>MPILEKAPQKMPVKASSWEELDLPKLPVPPLQQTLATYLQCMQHLVPEEQFRKSQAIVKRFGAPGGLGETLQEKLLERQEKTANWVSEYWLNDMYLNNRLALPVNSSPAVIFARQHFQDTNDQLRFAACLISGVLSYKTLLDSHSLPTDWAKGQLSGQPLCMKQYYRLFSSYRLPGHTQDTLVAQKSSIMPEPEHVIVACCNQFFVLDVVINFRRLSEGDLFTQLRKIVKMASNEDERLPPIGLLTSDGRSEWAKARTVLLKDSTNRDSLDMIERCICLVCLDGPGTGELSDTHRALQLLHGGGCSLNGANRWYDKSLQFVVGRDGTCGVVCEHSPFDGIVLVQCTEHLLKHMMTSNKKLVRADSVSELPAPRRLRWKCSPETQGHLASSAEKLQRIVKNLDFIVYKFDNYGKTFIKKQKYSPDGFIQVALQLA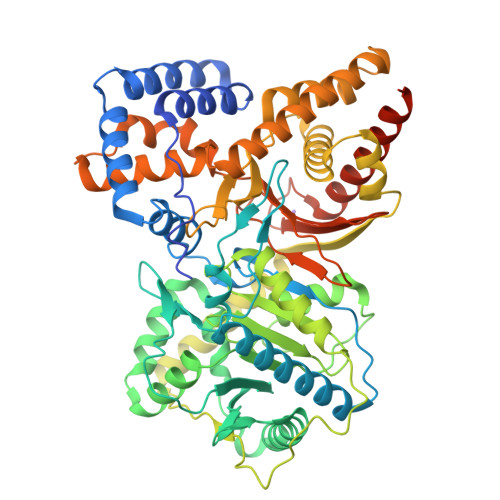YYRLYQRLVPTYESASIRRFQEGRVDNIRSATPEALAFVQAMTDHKAAMPASEKLQLLQTAMQAQTEYTVMAITGMAIDNHLLALRELARDLCKEPPEMFMDETYLMSNRFVLSTSQVPTTMEMFCCYGPVVPNGYGACYNPQPEAITFCISSFHSCKETSSVEFAEAVGASLVDMRDLCSSRQPADSKPPAPKEKARGPTKPSNLDSSH[2x]>NLSDDLSFNFDKFVPNQKNIIFQGDASVSTTGVLQVTKVSKPTTTSIGRALYAAPIQIWDSITGKVASFATSFSFVVKADKSDGVDGLAFFLAPANSQIPSGSSAGMFGLFSSSDSKSSNQIIAVEFDTYFGKAYNPWDPDFKHIGIDVNSIKSIKTVKWDWRNGEVADVVITYRAP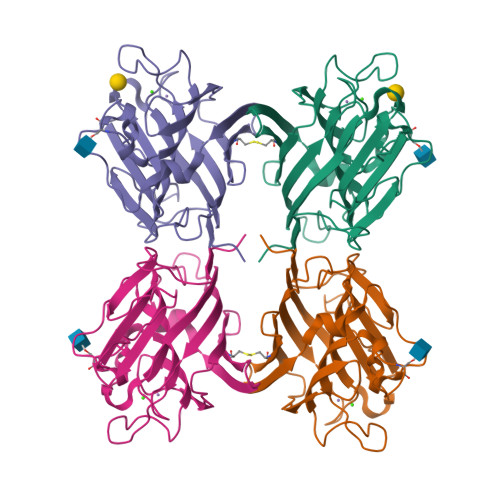TKSLTVCLSYPSDGTSNIITASVDLKAILPEWVSVGFSGGVGNAAEFETHDVLSWYFTSNLEANN[4x]>VMYYGKGDVFAYRTYLKPLTGVRTIPESPFSGRDHILFGVNVKISVGGTKLLTSFTKGDNSLVVATDSMKNFIQKHLASYTGTTIEGFLEYVATSFLKKYSHIEKISLIGEEIPFETTFAVKNGNRAASELVFKKSRNEYATAYLNMVRNEDNTLNITEQQSGLAGLQLIKVSGNSFVGFIRDEYTTLPEDSNRPLFVYLNIKWKYKNTEDSFGTNPENYVAAEQIRDIATSVFHETETLSIQHLIYLIGRRILERFPQLQEVYFESQNHTWDKIVEEIPESEGKVY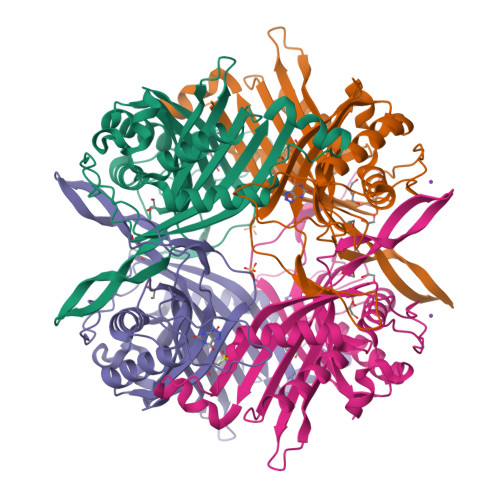TEPRPPYGFQCFTVTQEDLPHENIL[2x]> KPFKCSMCDYASVEVSKLKRHIRSHTGERPFQCSLCSYASRDTYKLKRHMRTHSGEKPYECYIC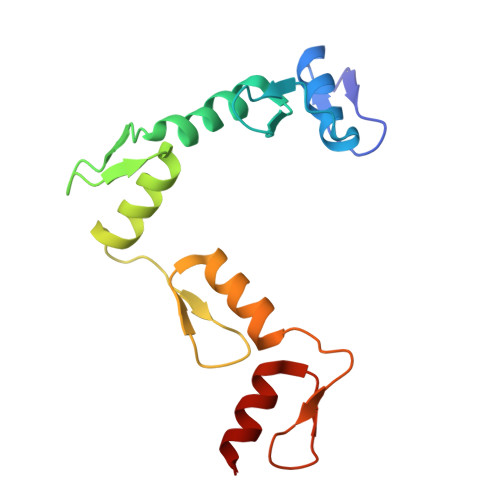HARFTQSGTMKMHILQKHTENVAKFHCPHCDTVIARKSDLGVHLRKQHSYIEQGKKCRYCDAVFHERYALIQHQKSH>MATRGANVIWFR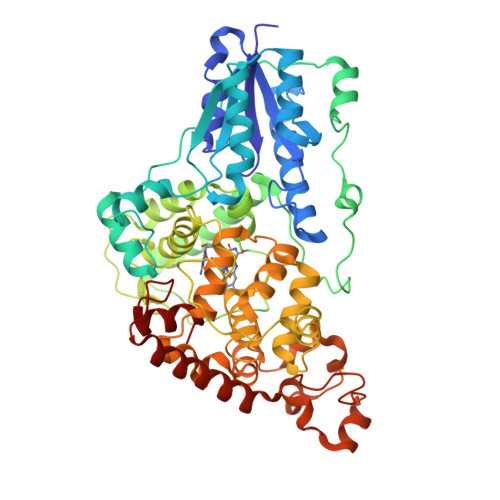HGLRLHDNPALLAALADKDQGIALIPVFIFDGESAGTKNVGYNRMRFLLDSLQDIDDQLQAATDGRGRLLVFEGEPAYIFRRLHEQVRLHRICIEQDCEPIWNERDESIRSLCRELNIDFVEKVSHTLWDPQLVIETNGGIPPLTYQMFLHTVQIIGLPPRPTADARLEDATFVELDPEFCRSLKLFEQLPTPEHFNVYGDNMGFLAKINWRGGETQALLLLDERLKVEQHAFERGFYLPNQALPNIHDSPKSMSAHLRFGCLSVRRFYWSVHDLFKNVQLRACVRGVQMTGGAHITGQLIWREYFYTMSVNNPNYDRMEGNDICLSIPWAKPNENLLQSWRLGQTGFPLIDGAMRQLLAEGWLHHTLRNTVATFLTRGGLWQSWEHGLQHFLKYLLDADWSVCAGNWMWVSSSAFERLLDSSLVTCPVALAKRLDPDGTYIKQYVPELMNVPKEFVHEPWRMSAEQQEQYECLIGVHYPERIIDLSMAVKRNMLAMKSLRNSLITPPPHCRPSNEEEVRQFFWLAD[2x]>MSVIVYRNNQSTLTLNGYTFQHLYQGAALVLTPVNAKTARTNSINGGVSISGRVDGGVHTLAIMVQKHSPDDKFLNDAKNSQEPVVFDGSMKRAYTESGTLKKATTTLETGSITTQPTKTDNNQDPDDSRTYVIEFRNSVETF[6x];>[6x]MSDFLNQYLLYLIKQYYEKPKANAEAQLLISTWETYADFIANFGNNFDIDNAEGEVLDLIGRILDLSRQVNDVIPASFFGFSENPLAKGFTSLENPLRVSAPFFKLTSKVYTDYQLTDTQYRKFLKVKAAKNICSPYLASDEKISLQQVVFDAFDGRAYVVDGKDQTLRLYVSPSIDDDELRLLINLDILPRPITFRYIIYGNAEPGVTFGFSNNPGSKSFGSLNNPSRQENGGVFARFYNG;>[6x]MSLVNGMVESLNNTKSETEIGIGGYRLFARVRETVNYRNIVPTDTLEDGSSSTDDIINEPITVSIEGVVSNLFVEERQYPQLVSRDFSAVGEITALLPAKSQQQIQRISQIDSQIRDAVLAAERAERLAGKPYEFFGNSGNSAKTEQEKFIDFMEALYFSRRPTEVSVNFRDYKNMALVSFIPVRDNNTKDTRFTADFQQINYSTLVYTPVSSPSKSVSGKVSDASNKGGQNPESNETGERSLLSSLVGG;>MNLIENITSEYIQTHALEFSRGFAVLTLIYEQAVQMWKMNVVYTRAGDEEPQPPIYGVKLALSTTHIKHRNWPFDFTVIDTTNNGMDPYRADDFETGRCQLYFITPEEMIQVRGVDVQ[6x];>MSLTFNENGVQTNTFSELRALLEAGYREIYGTDIVTDQESPDGQRINLETLLRFDIESAFSWLYSNLDPDLNTGDMQQIIGKLSGLVLLPASRSQWDVTINMSRAKTLPAGYTITDENNQNWFLDSDVDVLIGDNEVTFLSSLWGSISGISGSSFTQATPEIGVVSISASADAIQGREEETPEQFRLRRQRSTENPAQSTIGSIYAKLAQINGVTDLQVYDNSSDTPDQITGSSNPDILNGSEPVTIGAHTMWVVIEGGSLDDIGEVVAKHRLGNTKGSVQVSYIDTLTKPNGDDFQIVNLHNIDRPVLGDLYVRLTATQKVSGSPIDTDAIKNKLSLVDFEIGQYVDADALYQQSLITNSNYNVTDLEVSLNGIDWTDGRVFSGYDGKLSISTSNVTITTVPV[12x];>[6x]MASISEVIRVSLQQEGRAIAPDNMNAVGIITGNQGVLSTADRYRIYRTAAAVASDFGASSQESAFANTFFDTTPNPISAGGVLVIGYWRSASETVAATSATLVSEQTSESVLIPLLNAINDGSFTITVDGGTEQEVTALDFTGVSELSEVATILNSAITGATVSEDNGYFKVTSSTTGATSLLSYLGVATSGTDISAVLGMNSESGAVLTQGTDQVVLPAETKLEGITAIKSEVNIKGAMFIDQILDADIPGIASFAGANNMLVYEVFDTGYLSKNVSNPVWAVKLAGQSNFRCLLSKSGNRKFAATYMARMHTVLFSG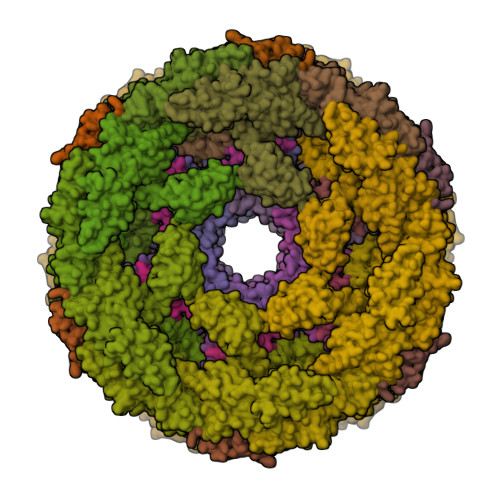QNTAITMQLKELSVTAEEYTDTEIANAKTVGLDLLTTIKNEQALLTSGANDFCDNVYNLEAFRDEIQTNNYNLLKTTSTKIPQTDPGMDTIEDDTEKTCEKYVRNGVFAPGTWTRSDFFGDRQQFVDAIAQKGYYVLIGDLADQTTAERQSRVSPVIQIAVKNAGAVHEEDIIISVNL;>[6x]MRVRTLDDNGDWTFGRGKADYITSKKAIAQTVSTRIKSWANDNPLAMNANIDWKDLLGRKGTEDTILREIERVVVQTDGVIRVTELEVIKTEKRVQSILLSYDTIYDDSETLEINDL> EVNVVMTGDMTTRLAFAGEQLKQALVEKGYEVNQTTDEKEIGGGKRSIYLNLLNDTTKKNKERFDISTKGKNTYVTGYDGNGIIYGCRELIDQLDQSGTMDFKPVSDAPEMVLRGACIGLQKTTYLPGHAVYEYPYTPESFPWFYDKERWIKYLDMMVENRMNSLYLWNGHPFASLVKLKDYPFALEVDEETFKKNEEMFSFLTTEAEKRGIFVIQMFYNIIVSKPFADHYGIKTQDRNRPITPLISDYTRKSVAAFIEKYPNVGLLVCLGEAIGTYEEDVEWFTKTIIPGIKDGLKVLG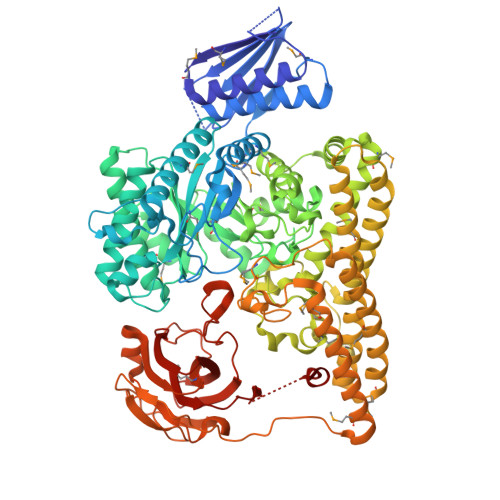RTDEPPVLVRAHDTDCKMVIDAALPLYKNLYTMHKYNGESLTTYEPRGPWAKIHKDLSSLGSVHISNVHILANLEPWRWSSPDFIQKSVKAMHSVHGANALHIYPQANYWDWPYTADKLANGEREEQVYRDWAWYKAWGRYAWKADRNRLEEIKYWDKQFGDFYGIPAEMADNIRIAYEESGEIAPKLLRRFGITEGNRQTLLLGMFMSQFVNPYKYTIHYGFYESCGPGGEKLIEYVEKEWKKQPHVGELPLDIINQVIEHGDKAVAAIDKVVSSAKKNSDELRRLQNDMHCYREYAYAFYYKVKAAQHVLNYHWGKNMDELDKAVPLMEESLKHYTKLVDLTKDTYLFANSMQTAQRRIPIGGDDGNNKTWSEMLVHYKAELYNFKENIEMLKDKKVRKCVEVTPLKEADVKILNNLTKVKIEKGAKIFSNIDGGIDAIAKEITGLTGFVFNGEKQRDDATTIEFECSSPVTMLVAYFKDDHRKFAKAPRLESDASANDYGQAEPVLTNALHVKGVALADIYPYKFKAGRHTLILPKGYCGVLGFTEDKIKERDVALEGGADAPDWLFY>ETGFVNKDQIAKDVKQFYDQALQQAVVDDDANNAKAVVKTFHETLDCCGSSTLTALTTSVLKNNLCPSGSNIISNLFKEDCHQKI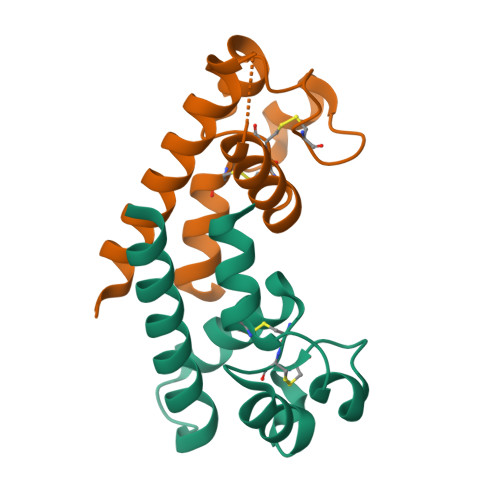DDLFSGKGTKHHHHHH[5x]> MQFHLNGFRPGNPLIAPASPLAPAHTEAVPSQVDVLIVGCGPAGLTLAAQLAAFPDIRTCIVEQKEGPMELGQADGIACRTMEMFEAFEFADSILKEACWINDVTFWKPDPGQPGRIARHGRVQDTEDGLSEFPHVILNQARVHDHYLERMRNSPSRLEPHYARRVLDVKVDHGAADYPVTVT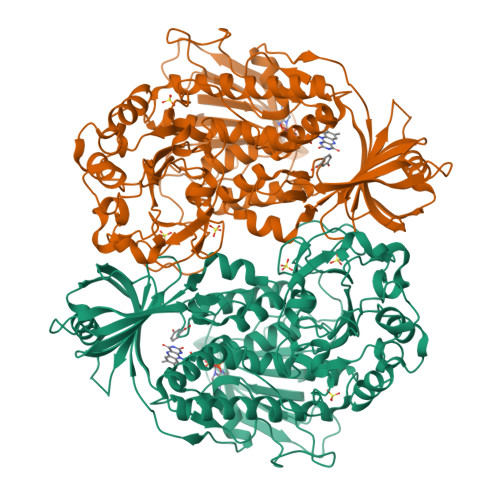LERCDAAHAGQIETVQARYVVGCDGARSNVRRAIGRQLVGDSANQAWGVMDVLAVTDFPDVRYKVAIQSEQGNVLIIPREGGHLVRFYVEMDKLDADERVASRNITVEQLIATAQRVLHPYKLEVKNVPWWSVYEIGQRICAKYDDVVDAVATPDSPLPRVFIAGDACHTHSPKAGQGMNFSMQDSFNLGWKLAAVLRKQCAPELLHTYSSERQVVAQQLIDFDREWAKMFSDPAKEGGQGGVDPKEFQKYFEQHGRFTAGVGTHYAPSLLTGQAKHQALASGFTVGMRFHSAPVVRVCDAKPVQLGHCGKADGRWRLYAFAAQNDLAQPESGLLALCRFLEGDAASPLRRFTPAGQDIDSIFDLRAVFPQAYTEVALETLPALLLPPKGQLGMIDYEKVFSPDLKNAGQDIFELRGIDRQQGALVVVRPDQYVAQVLPLGDHAALSAYFESFMRA>[2x]SNAMQIVKKEKFILKEYTFENGRTIPVQMGYETYGTLNRERSNVILICHYF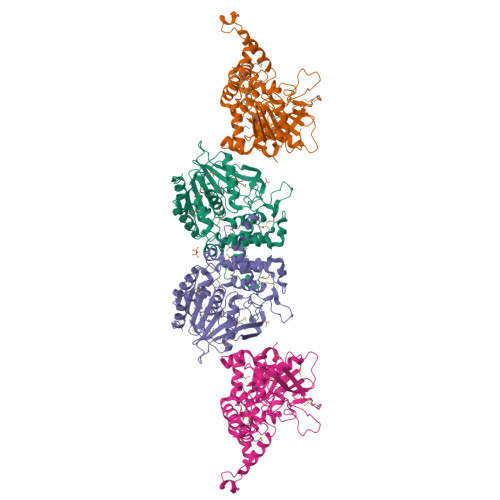SATSHAAGKYTAHDEESGWWDGLIGPGKAIDTNQYFVICTDNLCNVQVKNPHVITTGPKSINPKTGDEYAMDFPVFTFLDVARMQCELIKDMGIARLHAVMGPSAGGMIAQQWAVHYPHMVERMIGVITNPQNPIITSVNVAQNAIEAIRLDPSWKGGKYGEEQPMKGLQLANRMMFMNAFDEHFYETTYPRNSIEVEPYEKVSSLTSFEKEINKLTYRSIELVDANSWMYTAKAVLLHDIAHGFSSLEEALSNVEANVLMIPCKQDLLQPSRYNYKMVDLLQKQGKYAEVYEIESINGHMAGVFDIHLFEKKVYEFLNRKVSSFV> MSKSLQRALVFSGQGAHRRGMATEYLRIPAVACLWERMKGSMEQKYGISLQDIITENPTRLYVYNDAYDVAAICERSCQDGGSVVESTPKQKLISHPQGVLSLTSLTQPCMLAAHMVSLEYLKETRGYSVESSEVIAGHSLGEFSALCALGVLSPEVAIDLVYRRGALMEDAVKHSSQSNEGHLMFACNPQRAKLCVEDPDLAVDQLHIFVELIARNLSTTASFIEVVNYNISYEQYVVVGDPIALSALGKCLDPQFRATSCGSSATLDNIVRTAVSSVLQDKQEGITMNPNTGPAPDFVTSCARKY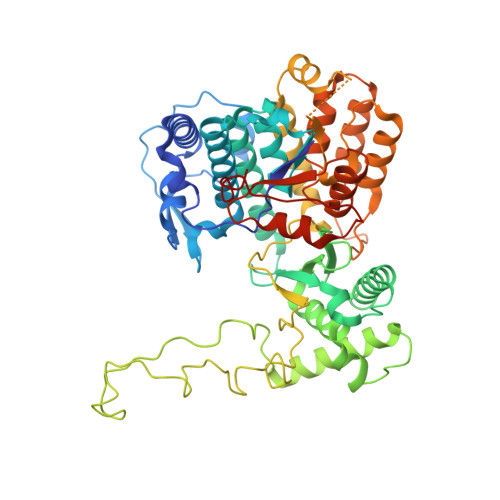GIRSTFRRFLRGPDDGYTPSLEELTHLTLQEDGRSGLKKKSWFIPLPLSIPFHSSMLRRAMDLFLPVVRDALPDEETMRSFFCIPQCGGSDXGPSSRCASEPKKPVWLTNLTGTAFRPFDVDFQRDALDAMQSMNVGEIRHNGRYHTNLVELAFKNGMDTSSVRDMCAAVLAAQLAHPVQWIDVMDSAVFQHGVREAHEISPVRTVADMFKRTVFRGKTSDASVGEAALDIVTRCLPSEERFL>[4x]TKPFTLPILTISELT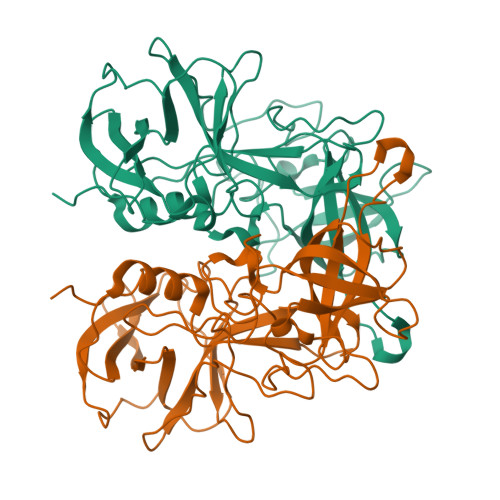NSRFPIPIEQLYTAPNENNVVQCQNGRCTLDGELQGTTQLLSSAVCSYRGRTVANSGDYWDQNLLQLTYPSGASYDPTDEVPAPLGTQDFSGILYGVLTQDNVSEGTGEAKNAKGVYISTTSGKFTPKIGSIGLHSITENVHPNQQSRFTPVGVAQNENTPFQQWVLPHYAGALALNTNLAPAVAPTFPGEQLLFFRSRVPCVQGLRGQDAFIDCLLPQEWVNHFYQEAAPSQADVALIRYVNPDTGRTLFEAKLHRSGFITVSHTGAYPLVVPPNGHFRFDSWVNQFYSLAPM>[8x]GMPYERKIINDPVFGFINIPKGLLYDIVRHPLLQRLTRIKQVGLSSVVYPGAQHTRFQHSLGAFYLMSEAITQLTSKGNFIFDSEAEAVQAAILLHDIGHGPFSHVLEDTIVQGVSHEEISLMLMER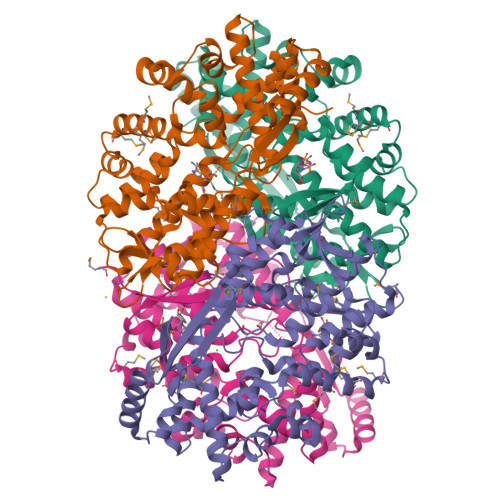MNKEMNGQLSLAIQIFKDEYPKRFLHQLVSGQLDMDRLDYLRRDSFYTGVTEGNIGSARIIKMLDVADDRLVIESKGIYSIENFLTARRLMYWQVYLHKTSVAYERMLISTLLRAKELASQGVELFASPALHFFLYNDINHTEFHNNPDCLENFIQLDDNDIWTALKVWSNHPDKVLSTLSLGMINRNIFKVENSAEPIGEDRIKELTLQISQQLGITLSEANYFVSTPSIEKNMYDPADDSIDIIYKDGTIKNIAEASDMLNISLLSKKVKKYYLCYQRLHR>MAMGDKAKLFRNISQRCLRRGSPEEALRFLKEWARHEKNDPEPLYQMGIALANLGDYQRAVTVFDKVLKLRPNHFMASYRKGAVLLKIKQYKLALPVLEAVVAAAPADARAYYLLGLAYDGDEQLEKGIEAMQKAVDLDP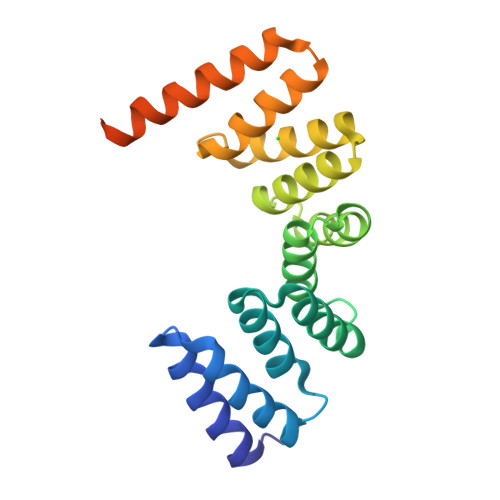EEIKYHQHLGFMNVRKDDHKTAAEHFTKVMELERSQDSDEEELALVPRGSSAHHHHHHHHHH[6x]>MGHHHHHHGGSENLYFQGNEDILKASATQSAVAGTYQIQVNSLATSSKIALQAIADPANAKFNSGTLNISVGDTKLPAITVDSSNNTLAGMRDAINQAGKEAGVSAT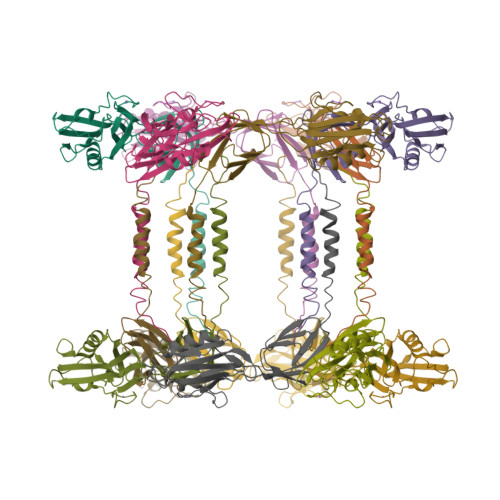IITDNSGSRLVLSSTKTGDGKDIKVEVSDDGSGGNTSLSQLAFDPATAPKLSDGAAAGYVTKAANGEITVDGLKRSIASNSVSDVIDGVSFDVKAVTEAGKPITLTVSRDDAGVKDNVKKFVEAYNTLTKFINEQTVVTKVGEDKNPVTGALLGDASVRALVNTMRSELIASNENGSVRNLAALGITTTKDGTLEIDEKKLDKAISADFEGVASYFTGDTGLAKRLGDKMKPYTDAQGI[2x]> MRALLPYLALYKRHKWMLSLGIVLAIVTLLASIGLLTLSGWFLSASAVAGVAGLYSFNYMLPAAGVRGAAITRTAGRYFERLVSHDATFRVLQHLRIYTFSKLLPLSPAGLARYRQGELLNRVVADVDTLDHLYLRVISPLVGAFVVIMVVTIGLSFLDFTLAFTLGGIMLLTLFLMPPLFYRAGKSTGQNLTHLRGQYRQQLTAWLQGQAELTIFGASDRYRTQLENTEIQWLEAQRRQSELTALSQAIMLLIGALAVILMLWMASGGVGGNAQPGALIALFVFCALAAFEALAPVTGAFQHLGQVIASAVRISDLTDQKPEVTFPDTQTRVADRVSLTLRDVQFTYPEQSQQALKGISLQVNAGEHIAILGRTGCGKSTLLQQLTRAWDPQQGEILLNDSPIASLNEAALRQTISVVPQRVHLFSATLRDNLLLASPGSSDEALSEILRRVGLEKLLEDAGLNSWLGEGGRQLSGGELRRLAIARALLHDAPLVLLDEPTEGLDATTESQILELLAEMMREKTVLMVTHRLRGLSRFQQIIVMDNGQIIEQGTHAELLARQGRYYQFKQGL;> MNKSRQKELTRWLKQQSVISQRWLNISRLLGFVSGILIIAQAWFMARILQHMIMENIPREALLLPFTLLVLTFVLRAWVVWLRERVGYHAGQHIRFAIRRQVLDRLQQAGPAWIQGKPAGSWATLVLEQIDDMHDYYARYLPQMALAVSVPLLIVVAIFPSNWAAALILLGTAPLIPLFMALVGMGAADANRRNFLALARLSGHFLDRLRGMETLRIFGRGEAEIESIRSASEDFRQRTMEVLRLAFLSSGILEFFTSLSIALVAVYFGFSYLGELDFGHYDTGVTLAAGFLALILAPEFFQPLRDLGTFYHAKAQAVGAADSLKTFMETPLAHPQRGEAELASTDPVTIEAEELFITSPEGKTLAGPLNFTLPAGQRAVLVGRSGSGKSSLLNALSGFLSYQGSLRINGIELRDLSPESWRKHLSWVGQNPQLPAATLRDNVLLARPDASEQELQAALDNAWVSEFLPLLPQGVDTPVGDQAARLSVGQAQRVAVARALLNPCSLLLLDEPAASLDAHSEQRVMEALNAASLRQTTLMVTHQLEDLADWDVIWVMQDGRIIEQGRYAELSVAGGPFATLLAHRQEEI

The ABC transporter CydDC plays a central role in the biogenesis of membrane-integrated and soluble cytochromes. Here, we used cellular, biochemical, structural and computational methods to characterize the structure and function of the heterodimeric bacterial ABC transporter CydDC. We provide multi-level evidence that CydDC is a heme transporter required for functional maturation of cytochrome bd, a pharmaceutically relevant drug target. Each subunit is composed of a membrane domain formed by six transmembrane α-helices (TMH), an N-terminal cytoplasmic elbow helix oriented parallel to the membrane plane and a cytoplasmic NBD.

The nucleotide and substrate-free, inward-facing conformation of CydDC IFasisolatedapo, obtained in as isolated conditions, exhibits canonical features of type IV ABC transporters. The successful determination of the IFasisolatedapo conformation was followed by a screen for substrate molecules binding to CydDC. Next, we analyzed the dynamics of heme placed near the lateral entry site of CydDC in the IFasisolatedapo state. Analysis of nonbonded interaction energies between heme and IFasisolatedapo shows that electrostatic interactions between K3D, K7D, K314D and R192D and the heme propionates play a key role in attracting heme toward the lateral entry site.> MSEFM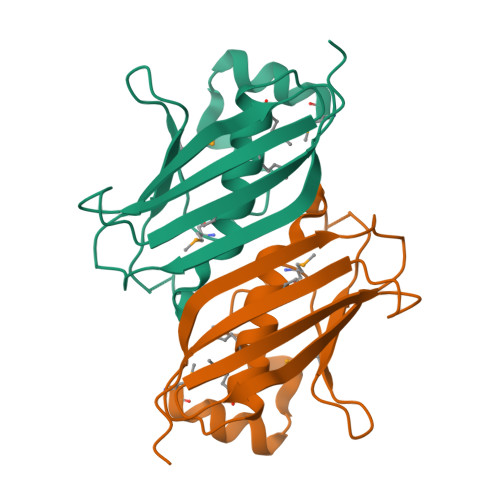QRFADLRDRKAYAEIVDALPYVKLMGTSMAEDEQGELRFELPFLQRNVGNTTLPALHGGLIGGFMESAAMIHLMWNRESLEAPKIVDFSLDYLRPGRPQTLFAQCEITKQGKRVAHVLIEAWQDDRSKPVAVARAHFLLTNLEHHHHHH>MRCFERYRVHLNRLSLSNAVMRMVSGYAPSVVGAMGWSIFSSGPAAAQSAGGGTDPATMVNNICTFILGPFGQSLAVLGIVAIGISWMFGRASLGLVAGVVGGIVIMFGA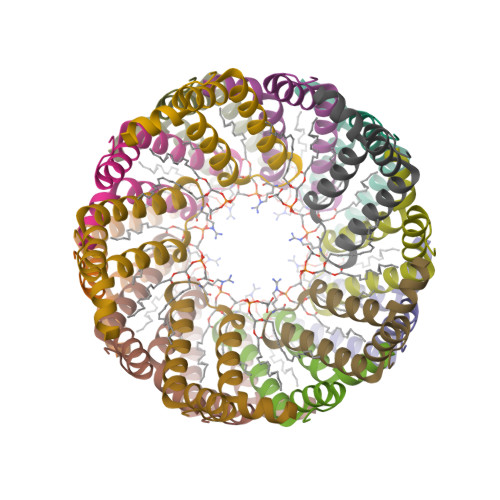SFLGKTLTGGG[15x]> MGHHHHHHADKGMTYSFDVRDNTLVVRRSTATKSGIKISYREDRGTSLLQKAFAGTEDEFWVELDQDVYVDKKIRKFLEEEKMKDMSTRVSGAVAAAIERSVEFDNFSKEAAANIEMAGVDDEEAGGSGL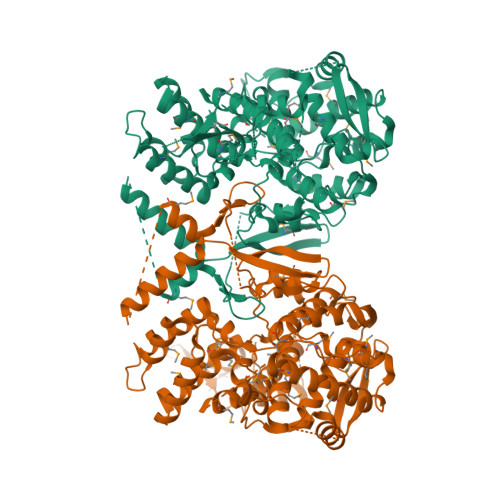VDNKRKNKGVSNMAYNLSLFIGMVFPALTTFFSAILSEGEMSIWQNGQAIMRILALADEDGKRQTRTGGQRVDMADVTKLNVVTANGKVKQVEVNLNDLKAAFRQSRPKRSDYRKGQGSKATESSISNQCMALIMKSVLSADQLFAPGVKMMRTNGFNASYTTLAEGANIPSKYLRHMRNCGGVALDLMGMKRIKNSPEGAKSKIFSIIQKKVRGRCRTEEQRLLTSALKISDGENKFQRIMDTLCTSFLIDPPRTTKCFIPPISSLMMYIQEGNSVLAMDFMKNGEDACKICREAKLKVGVNSTFTMSVARTCVAVSMVATAFCSADIIENAVPGSERYRSNIKANTTKPKKDSTYTIQGLRLSNVRYEARPETSQSNTDRSWQVNVTDSFGGLAVFNQGAIREMLGDGTSETTSVNVRALVKRILKSASERSARAVKTFMVGEQGKSAIVISGVGLFSIDFEGVEEAERITDMTP>[2x]MDYKDDDDKWSHPQFEKHHHHHHHHWSHPQFEKQPPPPGPLGDCLRDWEDLQQDFQNIQETHRLYRLKLEELTKLQNNCTSSITRQKKRLQELALALKKCKPSLPAEAEGAAQELENQMKERQGLFFDMEAYLPKKNGLYLSLVLGNVNVTLLSKQAKFAYKDEYEKFKLYLTIILILISFTCRFLLNSRVTDAAFNFLLVWYYCTLTIRESILINNGSRIKGWWVFHH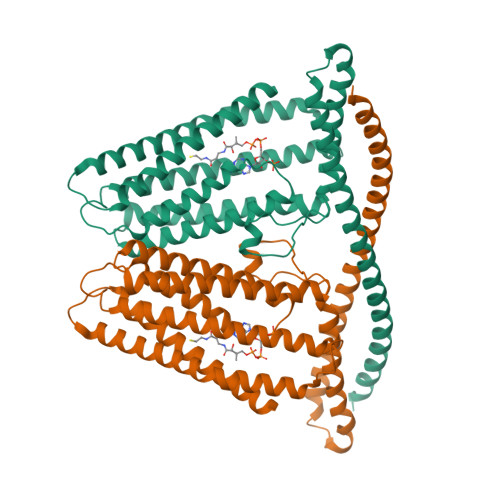YVSTFLSGVMLTWPDGLMYQKFRNQFLSFSMYQSFVQFLQYYYQSGCLYRLRALGERHTMDLTVEGFQSWMWRGLTFLLPFLFFGHFWQLFNALTLFNLAQDPQCKEWQVLMCGFPFLLLFLGNFFTTLRVVHHKFHSQRHGSKKD>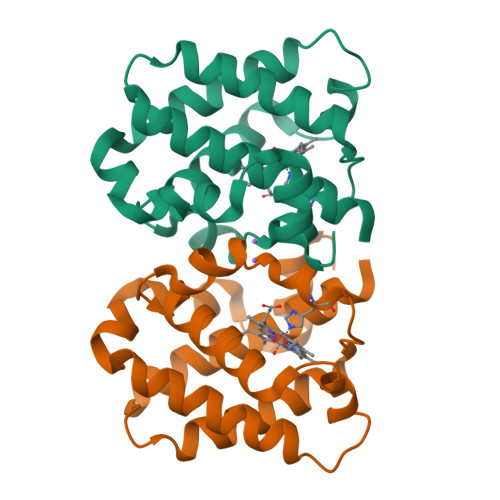 MQSLQDKASVLSGVDQAEAFAIDESNLFDKLGLQTFINLSTNFYTRVYDDEEEWFQSIFSNSNKEDAIQNQYEFFVQRMGGPPLYSQRKGHPALIGRHRPFPVTHQAAERWLEHMQNALDDSVDIDQDSKIKMMKFFRHTAFFLVAGNELKNQNEKPKHKPQCACKHAANKPAEE> IPAGIIPTGNVLSTIEVCIFFCIFDFFKQIRSDDNSLYSAQFDILLGTYCNTLNFVRFLELGLSVACICTKFPELAYVRDGVIQFEVQQPMIARDGPHPVDQPVHNYMVKRIHKRSLSAAFAIASEALSLLSNTYVAATEIDSSLRIRAIQQMARNLRTVSDSFERGTADQLLGVLLEKAPPLSLLSPINKFQPEGHLNRVARAALLSDLKRRVCADMFFMTRHAREPRLISAYLSDMVSCTQPSVMVSRITHTNTRGRQVDGVLVTTATLKRQLLQGILQIDDTAADVPVTYGEMVLQGTNLVTALVMGKAVRGMDDVARHLLDITDPNTLNIPSIPPQSNSDSTTAGLPVNARVPADLVIVGDKLVFLEALERRVYQATRVAYPLIGNIDITFIMPMGVFQANSMDRYTRHAGDFSTVSEQDPRQFPPQGIFFYNKDGILTQLTLRDAMGTICHSSLLDVEATLVALRQQHLDRQCYFGVYVAEGTEDTLDVQMGRFMETWADMMPHHPHWVNEHLTILQFIAPSNPRLRFELNPAFDFFVAPGDVDLPGPQRPPEAMPTVNATLRIINGNIPVPLCPISFRDCRGTQLGLGRHTMTPATIKAVKDTFEDRAYPTIFYMLEAVIHGNERNFCALLRLLTQCIRGYWEQSHRVAFVNNFHMLMYITTYLGNGELPEVCINIYRDLLQHVRALRQTITDFTIQGEGHNGETSEALNNILTDDTFIAPILWDCDALIYRDEAARDRLPAIRVSGRNGYQALHFVDMAGHNFQRRDNVLIHGRPVRGDTGQAIPITPHHDREWGILSKIYYYIVIPAFSRGSCCTMGVRYDRLYPALQAVIVPEIPADEEAPTTPEDPRHPLHAHQLVPNSLNVYFHNAHLTVDGDALLTLQELMGDMAERTTAILVSSAPDAGAATATTRNMRIYDGALYHGLIMMAYQAYDETIATGTFFYPVPVNPLFACPEHLASLRGMTNARRVLAKMVPPIPPFLGANHHATIRQPVAYHVTHSKSDFNTLTYSLLGGYFKFTPISLTHQLRTGFHPGIAFTVVRQDRFATEQLLYAERASESYFVGQIQVHHHDAIGGVNFTLTQPRAHVDLGVGYTAVCATAALRCPLTDMGNTAQNLFFSRGGVPMLHDNVTESLRRITASGGRLNPTEPLPIFGGLRPATSAGIARGQASVCEFVAMPVSTDLQYFRTACNPRGRASGMLYMGDRDADIEAIMFDHTQSDVAYTDRATLNPWASQKHSYGDRLYNGTYNLTGASPIYSPCFKFFTPAEVNTNCNTLDR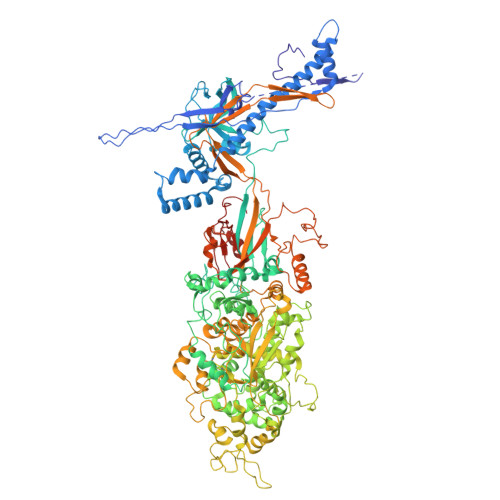LLMEAKAVASQSSTDTEYQFKRPPGSTEMTQDPCGLFQEAYPPLCSSDAAMLRTAHAGETGADEVHLAQYLIRDASPLRGCLPL>[3x]GPLGSAFQKCPICEKVIQG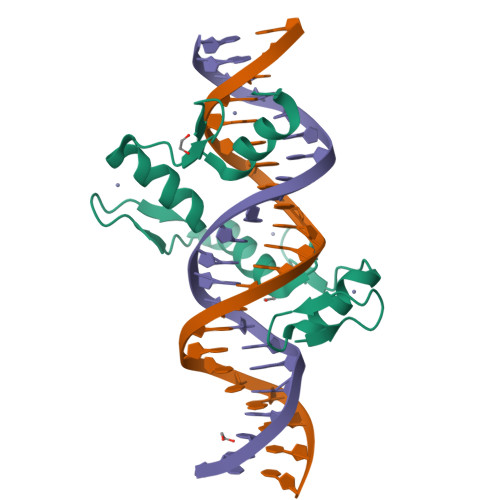AGKLPRHIRTHTGEKPYECNICKVRFTRQDKLKVHMRKHTGEKPYLCQQCGAAFAHNYDLKNHMRVHTGLRPYQCDSCCKTFVRSDHLHRHLKKDGCNGVPSRRGRKLERPHRD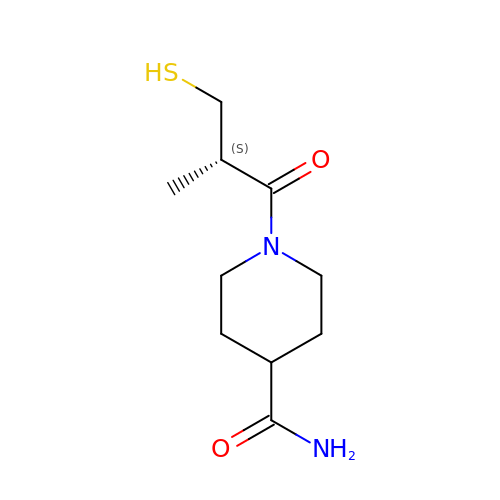1-[(2S)-2-methyl-3-sulfanyl-propanoyl]piperidine-4-carboxamide | C10 H18 N2 O2 S | OHKVCMUJTCAISN-SSDOTTSWSA-N>NLVQFSYLIQCANHGRRPTRHYMDYGCYCGWGGSGTPVDELDRCCKIHDDCYSDAEKKGCSPKMSAYDYYCGENGPYCRNIKKKCLRFVCDCDVEAAFCFAKAPYNNAN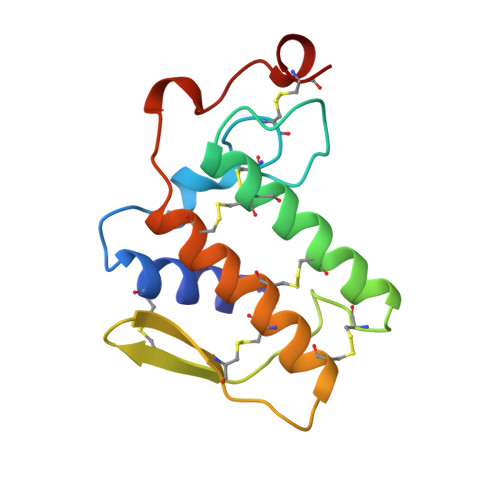WNIDTKKRCQ[2x]In this study, we purified three GAOR enzymes belonging to the XOR family, from the thermoacidophilic archaeon S. tokodaii. However, our biochemical data showed that in S. tokodaii, GAOR2 is more specific to GA, as compared with GAOR1, and indicated that GAOR2 is responsible for the GA oxidation in the npED glycolytic pathway in Sulfolobales. In summary, we isolated and characterized the three GAORs from S. tokodaii, and found that GAOR2 and GAOR3 share the same M/S-subunits but contain different L-subunits, and exhibit distinct substrate specificities. We determined the crystal structure of GAOR2, as the first structure of an archaeal Mo-containing hydroxylase, thereby providing insights into the subunit assembly and the substrate specificity of the three GAORs.

The asymmetric unit contains one hetero-trimer (LMS complex), one Mo-PCD (L-subunit), one FAD (M-subunit), two [2Fe-2S] clusters (designated as I and II) (S-subunit), and solvent molecules. The two hetero-trimers are related by crystallographic 2-fold symmetry to form a functional (LMS)2 dimer of GAOR2, where the L-subunits mediate the dimerization. GAOR2 has a butterfly-shaped, hetero-hexameric structure with a molecular size of approximately 140×65×90 Å, as observed for other XOR family enzymes. The Mo-PCD, [2Fe-2S] I, [2Fe-2S] II and FAD are located almost linearly, with distances of 13.4, 11.5 and 7.0 Å, respectively. In the GAOR2 structure, the Mo atom is penta-coordinated by two equatorial cis dithiolene sulfurs and three oxygen ligands: an apical oxo ligand (O1, 1.8 Å), a basal oxo ligand (O2, 1.9 Å), and a water molecule (OH, 2.4 Å). Although the present GAOR2 structure lacks a substrate, a polyethylene glycol molecule (pentaethylene glycol, C10H22O6) derived from the cyoprotectant solution is bound within a pocket formed by several residues in the L-subunit (Tyr190L, Ile219L, Asp292L, Asp293L, Gly296L, Asn297L, Ser330L, Arg336L, Phe417L and Gly483L). In the GAOR2 structure, Glu672L, a conserved catalytic Glu residue, is located at a position similar to those in other XOR family hydroxylases, such as DgAOR (Glu869) and bovine XOR (Glu1261), suggesting that the catalytic mechanism of GAOR2 is similar to those of other XOR family enzymes. The electron flow during the GAOR2 reaction is predicted as follows: electrons are depleted from the substrate aldehyde to Mo-PCD, and are then transferred via [2Fe-2S] I, [2Fe-2S] II and FAD to external electron acceptors, such as DCPIP and MV. Ala531 of DgAOR is also replaced with the hydrophilic Ser330L in GAOR2. These structural differences can explain why GAOR2 efficiently oxidizes hydrophilic glyceraldehyde, whereas DgAOR prefers aromatic aldehydes. There are four major L–M/S interfaces, and the key residues at the interface are highly conserved in the L-subunits of GAOR2 (STK23390) and GAOR3 (STK24840), consistent with the compatibility of the M/S-subunits between GAOR2 and GAOR3.

> MYIGKPIKRIEDLRLITGKGAYVDDIELPGTLFVAFVRSKYPHARIKVKKEEGIFTGEDINPGKDFPIATKETTYVGQPIAIVIAKDRYEAYDLIESVEVEYEELDYVLDPEKALEDKVKVHSGLSSNIYYHERWKGGDVEKAFKEADLTISDTLINQRVIASPLETRGALAYFDGNKLTFYSSTQSAHYLRRNLVDFLGFENIRVIQPDVGGAFGSKIIAHPEEYALAKLALMLRKPLKWVPTRTEEFISAGHGRDKKLKFEVAVKKDGTILGIRGTLIANLGAPYPDANDDESGNVKSTVRMLPGIYKIIGADIDAYAVHTNITPTQSYRGAGRPEGIYFIERIVNIVADELGIDQYEIRLKNAIDTLPYTNIFGVTYDSGNVKKLLEIGKKYYDELKKEDGCVGVSSYIEITAFGPWEVARISVKYDGKITLVTGTGPHGQGDATAFAQIAADVLELPIEKIEVRWGDTEIIEDGIGTWGSRTVTIGGSAVLLASQKLKDKLIEIGAKILNADKEEVEYKEGNVTHKKNGNKVTFNEIVKNAFKMGESLDTTAIYNVKQPPTTPYGVHLALVKVDGTGKVFVKKYVAVDDVGTVINPLLAEGQAIGGIVQGMAQALLEGAFFDENGQLLTTNFQDYPIPTAVEIPEKIDWYYEILGKSPHPTGSKGIGEAGAIAATPTIINAVEQCIKKRITKMPVKFEELVS;> MYPPKFGYVIPDNLNEALEFLEEHQDARPLAGGHSLIPMLKLRLIRPSYIVEIRRFSNLSYITKDGNLYKIGALTTHYNISKSSIPLLSETASNIGDPQVRNMGTIGGSISHLDPSADYPAALIAMDAKVKITSRKGDRVVNFKSFAKDMFTPDLNPGELVTEIQVPTFEGYKFSYQKLERRAGDFAIVGVALLLKLSGDVIEDVRIGLTAVNNVAVRAKGAEEELLGKRLNDEIIEKAATRAMESANPTSDLRGSAEYKKKMVKVLTKRAIITALKR;> MKIINSDQKVKITLKINGEKYETEVEPRRLLVHVLRELGFTGVHIGCDTSNCGACTVIMNGKSVKSCTVLAVEADGAEILTVEGLAKDGKLHPIQEAFWENHALQCGYCTPGMIMEAYWLLREKPNPTEEEIREGISGNLCRCTGYQNIVKAIKAAAEKLSQTPYQHQ Tom1p is a large, 374 kDa member of a broadly conserved family of HUWE1 factors (also called Mule, Lasu, Ureb1, Arf-BP1, HectH9/E3^Histone^, Ptr1, Upl1, or Eel-1;). This family is characterized by a large N-terminal domain attached to a smaller C-terminal HECT domain (Homologous to E6-AP Carboxyl Terminus) that provides ubiquitin ligase activity ([Fig fig1]). Tom1p has been implicated in the turnover of excess levels of small, basic proteins including ribosomal components and histones. We determined cryo-EM structures of Tom1p to reveal a helical repeat solenoid architecture for the 2,888 residues preceding the C-terminal HECT domain and an overall architecture that resembles the published structures of HUWE1 but with a larger fraction of ordered residues.

In addition to the closed ring structure, the Tom1p^His^ dataset contains particles in “intermediate” and “open” conformations that were reconstructed to resolutions of 7.79 and 7.10 Å, respectively ([Fig fig7], S6C-D). The distinction between closed and open/intermediate conformations is modeled as a rigid body hinging of 30° (open) or 15° (intermediate) centered at a loop (1316-1320) in the middle of the Body domain at the opposite side of the ring from the N-terminal Head and C-terminal HECT domains ([Fig fig7], 7C). The resolution does not allow precise modeling of the change in conformation, but apart from the rigid body rotations, conformational changes appear to be limited to some repacking of the interface between the two halves of the Body domain and modest shift in adjacent helices ([Fig fig7]). When aligned separately, the N-terminal and C-terminal halves of closed, intermediate, and open conformation Tom1 superimpose closely. The hinging motion, centered on loop 1316-1320 (green), is ^∽^ 15° and ^∽^30° for the intermediate and open conformations, respectively. Published cryo-EM studies of human HUWE1 indicated the presence of movement towards an open state analogous to that of Tom1p, although density for residues C-terminal to the hinge were not apparent. Our structural analysis revealed a closed solenoidal ring structure and multiple open conformations suggestive of dynamic conformational changes to a spiral shape. One possibility is that this ∼29 kDa domain occupies the solenoidal basket, perhaps extending above the basket rim, and that it retains basic substrate proteins in the central region of the solenoid. It is also possible that the shift from the closed ring to the open spiral form is important for function. Mutations expected to destabilize closure of the ring conformation were reported to compromise E3 ligase activity of human HUWE1 and similar mutations of *Nematocida* HUWE1 were found to destabilize the protein.

> MVLFTRCEKARKEKLAAGYKPLVDYLIDCDTPTFLERIEAIQEWDRSRDDLYVWIPILDRMDGLLLKVAEKYKYKQDPKKECEVKLVEMEAHDVDYCLKMLKFTRRLLLNTENRFVYSSGDVLMYLLNCPNFTIKLAVMRILAILGERFVIAREKIVAHNIFGDHNLRKKTLKLALSLSSSVMDEDGEHFSLVDLYFDKKKVPQKWRKLRFTHYTSNDFKKSSQQKNNINETQTSIKKVTMTTQELCEHSLQQIFDKGMALLPAESWFDFSIKASVAKAFSDDSGENIDLRNIIIETKLNAIAFVNTIFSPPQVSSKLFELDPYAFNSLTDLISLSETKIPKELRTDALFTLECISLKHVWCSDIIRNLGGNISHGLLFQILRYIAKTLREATDEIDEEYNVRFFYLISNLADVKPLHESLFAAGLIPTLLEIVSIRNCPYKRTLASATHLLETFIDNSETTTEFIENDGFTMLITSVANEIDFTLAHPETWQPPKYSVVYYSISFRELAYIRSLLKLVLKLLSTDSGDRIRNLIDSPILVSLKKILENKLVFGLTLITYTLDVVQKVINSEPTIYPVLVEAGLIPYVIDNFPKLIGPSAELLSLLPDVVSAICLNPEGLKQVKEKGLINNLFDFLLDADHARILTGGDRSTEYGTDIDELARHYPDLKANIVEALCNVIRKMPSTFRNEREFLFTSPKDQKYFFHRKNEEILTDKEEHEPAYWELLDKGTMLDTFTSVLFGMSLGNGSFSQVPQHLEARDFLAIIFMENPPYEYFTSVAISNVTEVLQYLDEKYEDYAFMDVMKVLNDQLENLNDFLNSPNDRSFFLERDGENSVRSCHSKLCRLAAILNIVTNVYIDLTTLSCKRIMQIYSYFDKRGFSLIKNLKLLFQKCALEEMYIRQHMPDSVITETMPLPIVDVSGDGPPLQIYIDDPKKGDQKGKITSVKTRNTLQMRTILYTLQSNTAILFRCFLRLSHSRNMDLEHKDLTTEVHIFENVVENVIEMLKATELEGHLPYILVLLNFNTFVFTIPKASPNSTEILQTIPAYIFYQKGGYLLYLHIIRDLFTRMTKIKSGGGGGGSRHHHHHHHHHHHHDLSSLDNINYIDESNGILTLSCLINALTFYNKSMQTETMENVQSIGKYYVSIDDDYNIMKALTVPIKVMALAMILDLDKSDSLFKTQSRNVPYSVFKQLLSMLKNIFTNVNIYTKELYELHWDLIFPPIKKISLFEQVGIPGDVAANYLTDTGDDLPADNSIGLFSPEQWEKYKKLIGEDKSIYYPQPMQAQYYKGCSSKELDELRDTFFNDGLPSRIFTVLPFYPKLVNAFAKTLLQIFTKYDEPTEVFAGRILDRILETDLDDPATLSSLIHLFGIFLNEKYIYQKASHLMQRFIEYLEKSLKPEHVNTPWFSKALYVYEIILAKSELPHLEELSKDVLLRYPLLSMAKVFRIPDPMKQKLFDILIRVSDISNFYSALATSRILIFYSRDELYANNIARSGILSRLLKVIGSFQKLDKINFLESSFLLLTRRCFETTENVDALIRAEINRSFTARPLGGGDDAVRELTTILEEKAHVVMRSPSQFIDVLCETARFHEFDDQGALVDYSLKRFLGEKDKNTQASSTEKSDIYERTGIMHLLLSQLMAASEKDWLSEPANSSDLPENKKAQLDPSRNPVCAYMIFLLKLLVELVSSYNQCKFEFLTFSRRNTYAERPRPRTTAINFFLYRLLDKPVGTDHDKHEAKRREVIGMLARSVIIGFLATVQDDRTTKTDVKLADPHMNFIRKFAIEAIIKAIRNATSSSKLLESNHLKLDMWFRIITSMVYVQAPYLRQLLDSNKVEADQYQLCKLVIDLGLPSVITEAMASIDLNYPFSKKIFNVAVEALNTISSTRNNFSEHFKIEDHDEVEDEVDESDKEEIPDMFKNSALGMYDVEDIEEDDDDDTSLIGDDDAMAFVDSDNGFEVVFSDEDDDMGEEDADDARSDSEENELSSEMQSSTADGTDVDYEVDDADGLIINIDQPSGDDEEMADYDANISHSSHSENEDDASMDVIEVYDDELSSGYDVDLSDYDVDESDWDSGLSSLSISDEDSESSEDEPINSTRMGDSRRRWLIAEGVELTDDSQGESEEDDRGVFRGIEHIFSNENEPLFRVHDEMRHRNHHRSINRTHFHSAMSAPSLSLLNRGRRNQSNLINPLGPTGLEQVENDISDQVTVAGSGSRPRSHHLHFSEVLVSGSFFDEPVLDGIILKSTVSRWKDIFDMFYDSKTYANCIIPTVINRLYKVSLALQKDLENKREQEKLKNKNLLFNEAKVESHNSSDAISVEQDDIQESNVTHDDHEPVYVTIQGSEVDIGGTDIDPEFMNALPDDIRADVFAQHVRERRAEARLNSDHNVHSREIDSDFLEAIPEDIREGILDTEAEEQRMFGRIGSSADVIRADDDVSNNDEEVENGLDHGNSNDRNNADPEKKKPARIYFAPLIDRAGIASLMKSVFISKPYIQREIYHELFYRLCSSKQNRNDLMNTFLFILSEGIIDQHSLEKVYNIISSRAMGHAKTTTVRQLPSDCTPLTVANQTIEILQSLIDADSRLKYFLIAEHDNLIVNKANNKSRKEALPDKKLRWPLWHLFSLLDRKLITDESVLMDLLTRILQVCTKTLAVLSTSSNGKENLSKKFHLPSFDEDDLMKILSIIMLDSCTTRVFQQTLNIIYNLSKLQGCMSIFTKHLVSLAISIMSKLKSALDGLSREVGTITTGMEINSELLQKFTLPSSDQAKLLKILTTVDFLYTHKRKEEERNVKDLQSLYDKMNGGPVWSSLSECLSQFEKSQAINTSATILLPLIESLMVVCRRSDLSQNRNTAVKYEDAKLLDFSKTRVENLFFPFTDAHKKLLNQMIRSNPKLMSGPFALLVKNPKVLDFDNKRYFFNAKLKSDNQERPKLPITVRREQVFLDSYRALFFKTNDEIKNSKLEITFKGESGVDAGGVTREWYQVLSRQMFNPDYALFLPVPSDKTTFHPNRTSGINPEHLSFFKFIGMIIGKAIRDQCFLDCHFSREVYKNILGRPVSLKDMESLDPDYYKSLVWILENDITDIIEETFSVETDDYGEHKVINLIEGGKDIIVTEANKQDYVKKVVEYKLQTSVKEQMDNFLVGFYALISKDLITIFDEQELELLISGLPDIDVDDWKNNTTYVNYTATCKEVSYFWRAVRSFDAEERAKLLQFVTGTSKVPLNGFKELSGVNGVCKFSIHRDFGSSERLPSSHTCFNQLNLPPYESYETLRGSLLLAINEGHEGFGLA> ASDTAVSNVVNYSTDVIYQIVTDRFVDGNTSNNPTGDLYDPTHTSLKKYFGGDWQGIINKINDGYLTGMGVTAIWIPQPVENIYAVLPDSTFGGSTSYHGYWARDFKRTNPYFGSFTDFQNLINTAHAHNIKVIIDFAPNHTSPASETDPTYAENGRLYDNGTLLGGYTNDTNGYFHHYGGTDFSSYEDGIYRNLFDLADLNQQNSTIDSYLKSAIKVWLDMGIDGIRLDAVKHMPFGWQKNFMDSILSYRPVFTFGEWFLGTNEIDVNNTYFANESGMSLLDFRFSQKVRQVFRDNTDTMYGLDSMIQSTASDYNFINDMVTFIDNHDMDRFYNGGSTRPVEQALAFTLTSRGVPAIYYGTEQYMTGN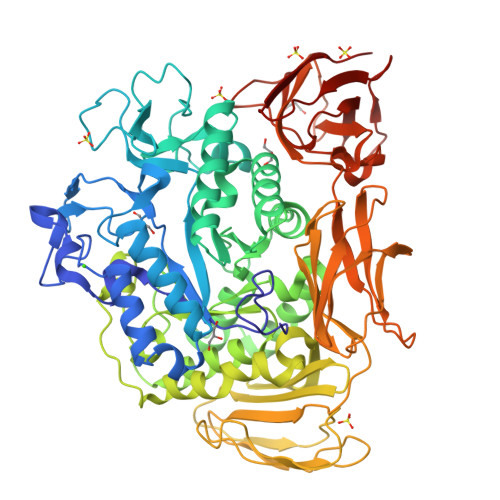GDPYNRAMMTSFNTSTTAYNVIKKLAPLRKSNPAIAYGTTQQRWINNDVYIYERKFGNNVALVAINRNLSTSYNITGLYTALPAGTYTDVLGGLLNGNSISVASDGSVTPFTLSAGEVAVWQYVSSSNSPLIGHVGPTMTKAGQTITIDGRGFGTTSGQVLFGSTAGTIVSWDDTEVKVKVPSVTPGKYNISLKTSSGATSNTYNNINILTGNQICVRFVVNNASTVYGENVYLTGNVAELGNWDTSKAIGPMFNQVVYQYPTWYYDVSVPAGTTIQFKFIKKNGNTITWEGGSNHTYTVPSSSTGTVIVNWQQ>MGSSHHHHHHSSGRENLYFQGMRAILFDVFGTLVDWRSSLIEQFQALERELGGTLPCVELTDRWRQQYKPAMDRVRNGQAPWQHLDQLHRQSLEALAGEFGLALDEALLQRITGFWHRLRPWPDTLAGMHALKADYWLAALSNGNTALMLDVARHA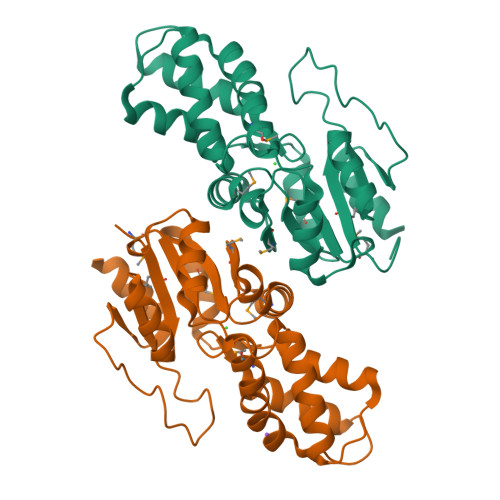GLPWDMLLCADLFGHYKPDPQVYLGACRLLDLPPQEVMLCAAHNYDLKAARALGLKTAFIARPLEYGPGQSQDLAAEQDWDLIASDLLDLHRQLAASA[4x]>MHHHHHHHHHHHHMMESGAPICHTCGEQVGHDANGDLFVACHECNYHICKSCFEYEIKEGRKVCLRCGSPYDENLLDDVEKKGSGNQSTMASHLNNSQDVGIHARHISSVSTVDSEMNDEYGNPIWKNRVESWKDKRNKKKKSNTKPETEPAQVPPEQQMENKPSAEASEPLSIVYPIPRNKLTPYRAVIIMRLIILGLFFHYRITNPVDSAFGLWLTSVICEIWFAFSWVLDQFPKWKPVNRETFIERLSARYEREGEPSQLAAVDFFVSTVDPLKEPPLITANTVLSILAVDYPVDKVSCYVSDDGAAMLTFESLVETAEFARKWVPFCKKFSIEPRAPEFYFSQKIDYLKDKVQPSFVKERRAMKRDYEEYKVRVNALVAKAQKTPDEGWTMQDGTPWPGNNTRDHPGMIQVFLGNTGARDIEGNELPRLVYVSREKRPGYQHHKKAGAENALVRVSAVLTNAPYILNLDCDHYVNNSKAVREAMCILMDPQVGRDVCYVQFPQRFDGIDRSDRYANRNIVFFDVNMKGLDGIQGPMYVGTGCVFNRQALYGYGPPSMPRLRKGKESSSCFSCCCPTKKKPAQDPAEVYRDAKREDLNAAIFNLTEIDNYDDYERSMLISQLSFEKTFGLSPVFIESTLMENGGVPESANSSTLIKEAIHVIGCGFEEKTEWGKEIGWIYGSVTEDILSGFKMHCRGWRSIYCMPVRPAFKGSAPINLSDRLHQVLRWALGSVEIFFSRHCPFWYGYGGGRLKWLQRLAYINTIVYPFTSLPLIAYCTIPAVCLLTGKFIIPTLSNLAS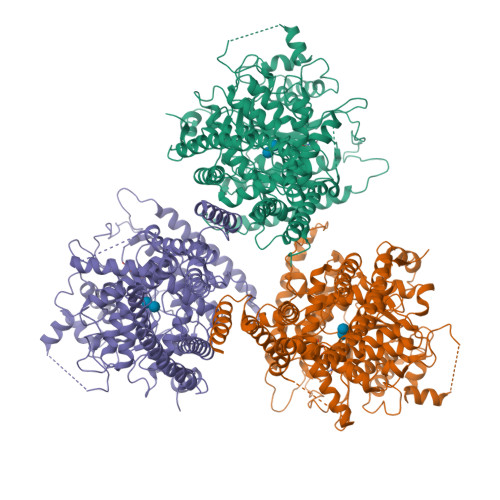MLFLGLFISIIVTAVLELRWSGVSIEDLWRNEQFWVIGGVSAHLFAVFQGFLKMLAGIDTNFTVTAKAADDTEFGELYMVKWTTLLIPPTTLLIINIVGVVAGFSDALNKGYEAWGPLFGKVFFAFWVILHLYPFLKGLMGRQNRTPTIVVLWSVLLTSVFSLVWVKINPFVNKVDNTLAGETCISIDC[3x]>MSLKKILIIDQQDFSRIELKNFLDSEYLVIESKNEKEALEQIDHHHPDLVILDMDIIGENSPNLCLKLKRSKGLKNVPLILLFSSEHKEAIVNGLHSG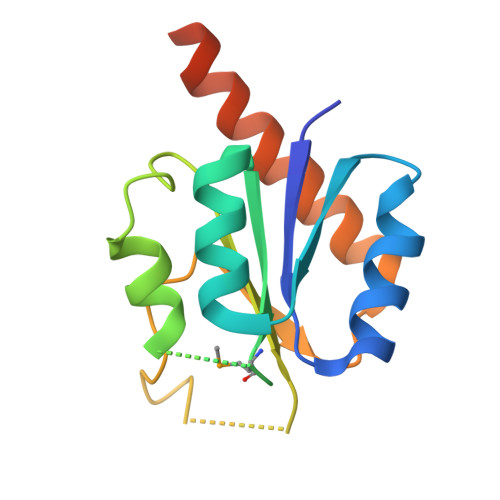ADDYLTKPFNRNDLLSRIEIHLRTQNYYSDLRKNEGHHHHHH[2x]>MSLSDQEFDEKYLELSEELKQSEKHKGTLDQGASQFLNAIEFVLRVYRQTEVIYVYAHLKNDQDTGNTDYQALYARASSLFSKVSEAVSWFEPEILQLSDDQIWQYFKEEPKLEVYRHYIQQIVDNRAHVLSAEQESLLAGAGEIFDASSDTFAVLNNADLVFPTIEGENGEIVQLSHGVYGQLLESTDRRVREAAFKGLYSVYEQFRNTFASTLGTHIKGHNFKAKVRNYSSAREASLSNNHIPESVYDTLVDVVNKHLPLLHRYMELRKRLLEVEKLHMYDLYTPVLGEAPITFTYEEAKEKALEALKPMGEEYMAIVEKAFSERWIDVVENKGKRSGAYSSGSYDTNPYILLNWHDTLDQLFTLVHEMGHSVHSYFTRSNQPYVYGDYSIFLAEIASTTNENILTEYLLETEKDPRVRAYVLNHYLDGFKGTVFRQTQFAEFEHFMHTEDEKGVPLTSEYLSDSYGKLNAKYYGPAVEEDPEIKFEWSRIPHFYYNYYVFQYSTGFSAASALAKKILNQEPEALENYLAYLKAGNSDYPVEVMKKAGVDMTQAAYIEDAMSMFEQRLNELEEL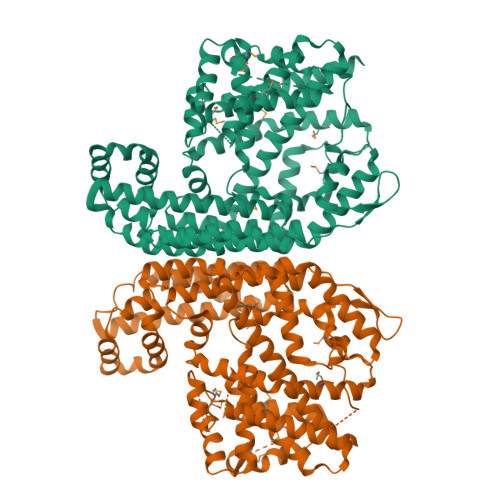IDREGHHHHHH[2x]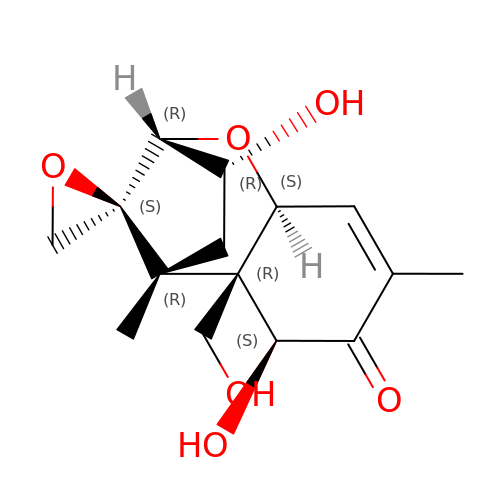(3alpha,7alpha)-3,7,15-trihydroxy-12,13-epoxytrichothec-9-en-8-one | C15 H20 O6 | LINOMUASTDIRTM-BGQOOYBISA-N>[4x]KDFLNPKYTLENFIVGEGNRLAYEVVKEALENLGSLYNPIFIYGSVGTGKTHLLQAAGNEAKKRGYRVIYSSADDFAQAMVEHLKKGTINEFRNMYKSVDLLLLDDVQFLSGKERTQIEFFHIFNTLYLLEKQIILASDRHPQKLDGVSDRLVSRFEGGILVEIELDNKTRFKIIKEKLKEFNLELRKEVIDYLLENTKNVREIEGKIKLIKLKGFEGLERKERKERDKLMQIVEFVANYYAVK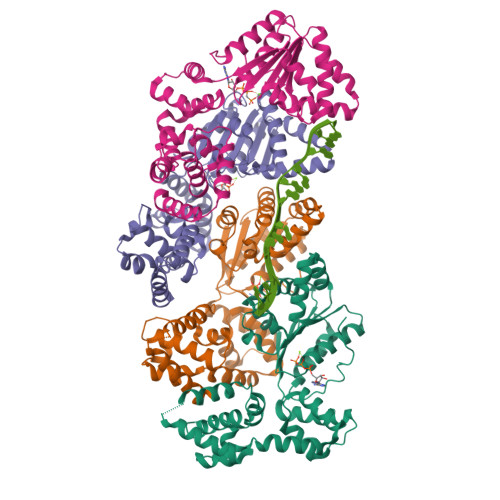VEDILSDKRNKRTSEARKIAMYLCRKVCSASLIEIARAFKRKDHTTVIHAIRSVEEEKKKDRKFKHLVGFLEKQAFDKIC> KMLNIKEYKEKLLSTLGEFLEDHFPLPDRSVKKKKKNIQESSVNLITLHEMLEILINRLFDVPHDPYVKISDSFWPPYVELLL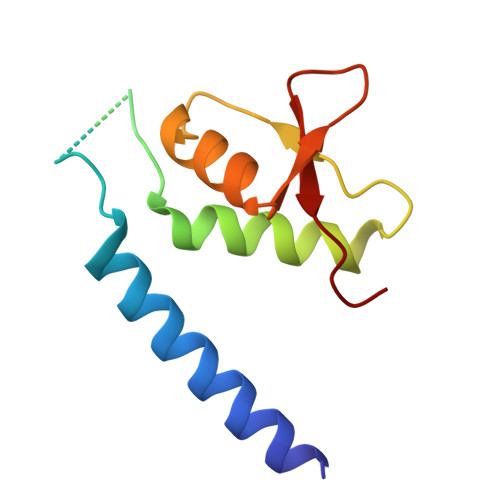RNGIALRHPEDPTRIRLEAFHQ> MWEGAIPLKHERVLNGGVATRVVKKTYSHPPEIHPTNLSFNDIDSMYCLGNDELIKYFPEGVGGKMMQLMPPGHPRGFLYRKQSHLLNCFIDKLPFWQSKEKALRSLTNGRPGFIMDGPTGCGKSALLCQAVHYARSRDIITLYIANAKAWTHGEWCWPSTILPGFFDAPDAAREFLRTVAEANGSLLQAWELRVTPQDLPLEQGEKQPRSLYDLCEWGHRAVAPASIDRQSVCIKFFFDEIRAEKTKPIIIAVDGWNLFSHETHFRYPHPDFLRTLTTLNDGLTDVDLYPQELPRIPASRLSFVRGLNKLILSKQDPNKFFITCTTRDFKPFDGVSGFADVENDRFKNSLDEYAPYDPEKDSFFHPMQVENFTEYEYRAFLRFAINSGE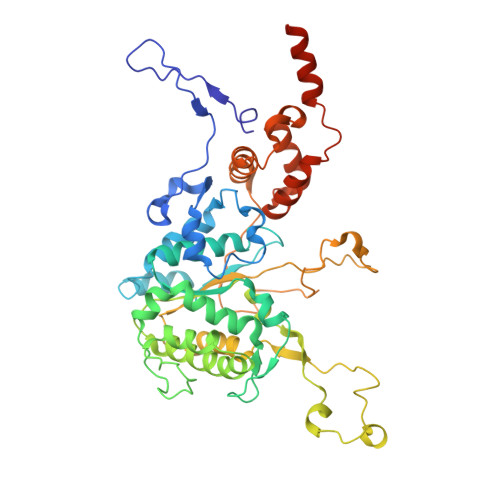LAGLGWGPMWHYSSDFERKLYKIDFMSDRNPQRVVDHYHQELVWRYEYKRTRQKQYLLARRKMWQGAEVSNPLRNGK> MDNKPETSLDNPVHQRSEPGSETGSSLSTITTHHLTVPPGLTPEEFQELSSSIAEFHSYRINPGQCSSLLAQRIHAPVETVWTVVRRFDKPQTYKHFIKSCSVGEDFRMTVGSTRDVTVISGLPAATS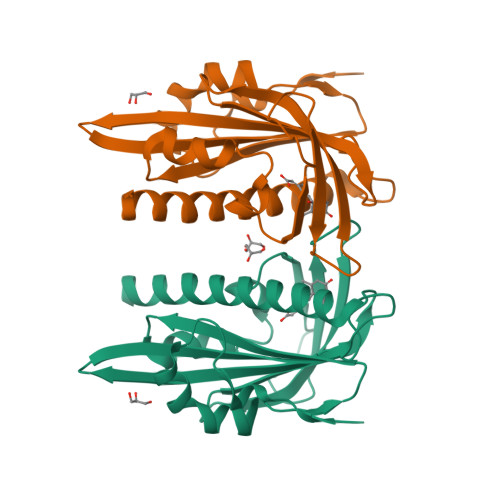TERLDILDDDRHVTGFSIIGGDHRLRNYRSVTTVHGFERDGEIWTVVLESYVVDVPEGNTEEDTRLFADTVVKLNLQKLASVTETLAREAGNGSVNSRDASHRS> MDRSGFGEISSPVIREAEVTRTARKQSAQKRVLLQASQDENFGNTTPRNQVIPRTPSSFRQPFTPTSRSLLRQPDISCILGTGGKSPRLTQSSGFFGNLSMVTNLDDSNWAAAFSSQRSGLFTNTEPHSITEDVTISAVMLREDDPGEAASMSMFSDFLQSFLKHSSSTVFDLVEEYENICGSQVNILSKIVSRATPGLQKFSKTASMLWLLQQEMVTWRLLASLYRDRIQSALEEESVFAVTAVNASEKTVVEALFQRDSLVRQSQLVVDWLESIAKDEIGEFSDNIEFYAKSVYWENTLHTLKQRQLTSYVGSVRPLVTELDPDAPIRQKMPLDDLDREDEVRLLKYLFTLIRAGMTEEAQRLCKRCGQAWRAATLEGWKLYHDPNVNGGTELEPVEGNPYRRIWKISCWRMAEDELF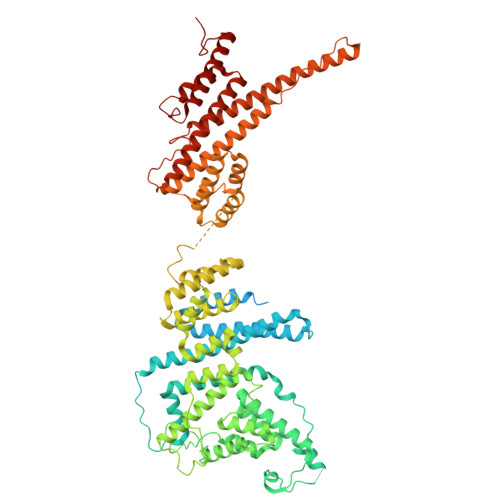NRYERAIYAALSGNLKQLLPVCDTWEDTVWAYFRVMVDSLVEQEIQTSVATLDETEELPREYLGANWTLEKVFEELQATDKKRVLEENQEHYHIVQKFLILGDIDGLMDEFSKWLSKSRNNLPGHLLRFMTHLILFFRTLGLQTKEEVSIEVLKTYIQLLIREKHTNLIAFYTCHLPQDLAVAQYALFLESVTEFEQRHHCLELAKEADLDVATITKTVVENIRKKDNGEFSHHDLAPALDTGTTEEDRLKIDVIDWLVFDPAQRAEALKQGNAIMRKFLASKKHEAAKEVFVKIPQDSIAEIYNQCEEQGMESPLPAEDDNAIREHLCIRAYLEAHETFNEWFKHMNSVPQKPALIPQPTFTEKVAHEHKEKKYEMDFGIWKGHLDALTADVKEKMYNVLLFVDGGWMVDVREDAKEDHERTHQMVLLRKLCLPMLCFLLHTILHSTGQYQECLQLADMVSSERHKLYLVFSKEELRKLLQKLRESSLMLLDQGLDPLGYEIQL>MLGLKTSIIGRRVIYFQEITSTNEFAKTSYLEEGTVIVADKQTMGHGALNRKWESPEGGLWLSIVLSPKVPQKDLPKIVFLGAVGVVETLKEFSIDGRIKWPNDVLVNYKKIAGVLVEGKGDKIVLGIGLNVNNKVPNGATSMKLELGSEVPLLSVFRSLITNLDRLYLNFLKNPMDILNLVRDNMILGVRVKILGDGSFEGIAEDIDDFGRLIIRLDSGEVKKVI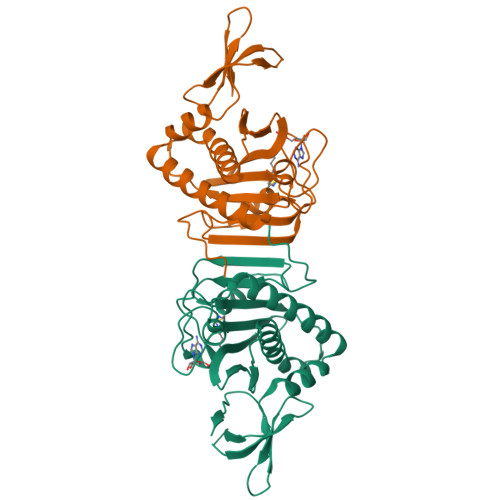YGDVSLRFL[2x]> MMQRCSTSLSRLCFRRLLRTPLLVYSIPPTRDVPSGIAHCPLSCSMRMVTSSNDDEFVFDPTLSIQKDAAIHTAKKSFETIVLEYVPAHAPEEARQKVKSYLTQHPIDILI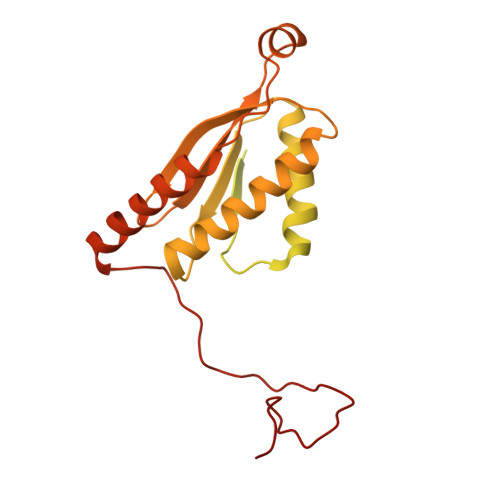TQPKVQITHLEDAESGAETKVSLSPCDLPEALQQARERGMNLVQMGARGDVAYCRIRRESTRILSLIHTELEALREQEEKQQGKGRGGVQAAAKMGELIDHTFRDAVDAHFVGWRSKKIVEDIRRRHPVKLTIKEFQSPECAIGKLREMCQAMQHYAQEKVIYHHFTSIVANDREASITFAPALPMAKSDSWKHIKYPGEKEWTNALRRMEDACRKSGRYGTYAKSNKLKLRSLGQTSYRVDKYGRKMD>[4x]MTTQPQLKENLTQWEYLALNSELNIADGHARQALSPGQQKIVNELPVLWAESEQRPVQQIESEAHQAYFTLLGQHGYPAEPGRVLSCYSSSVSMEILARSLSASVDRVALVHPTFDNIADLLRGNGLDLVPVEEDALHGADLSAELLSSVGCVFVTTPNNPTGRVLAEERLRRLAEQCAEHGT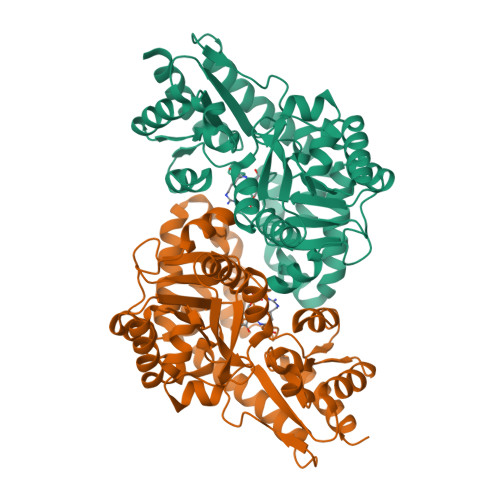VLALDTSFRGFDAAAHYDHYAVLQEAGCRWVVIEDTGKLWPTLDLKAGLLVFSEDIGLPVEKIYSDILLGVSPLILALIREFSRDAADGGLADLHAFILHNRSVVRRALAGVEGVSFPDPESRSSVERVAFAGRTGTEVWEELQRHHVFALPCRQFHWAEPSDGDHMVRIALSRSTEPLEKSVQVLRTVLETR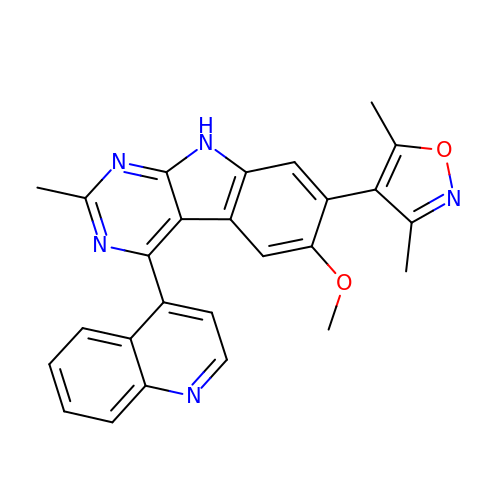7-(3,5-dimethyl-1,2-oxazol-4-yl)-6-methoxy-2-methyl-4-(quinolin-4-yl)-9H-pyrimido[4,5-b]indole | C26 H21 N5 O2 | AEANZCXROGPSBY-UHFFFAOYSA-N> MGPSLDFALSLLRRNVRQVQTDQGHFTMLGVRDRLAVLPRHSQPGKTIWIEHKLVNILDAVELVDEQGVNLELTLITLDTNEKFRDITKFIPENISTASDAT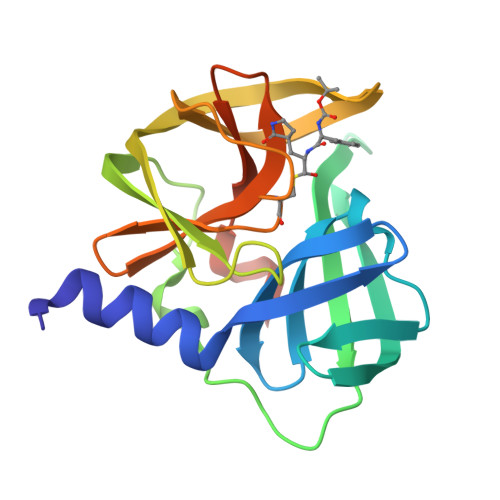LVINTEHMPSMFVPVGDVVQYGFLNLSGKPTHRTMMYNFPTKAGQCGGVVTSVGKVIGIHIGGNGRQGFCAGLKRSYFASEQLEHHHHHH> GMFNT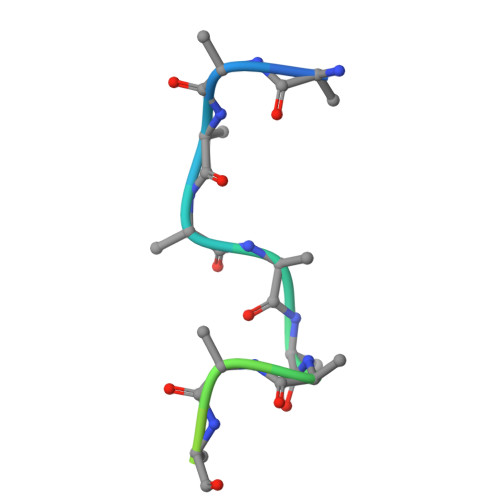TTMDDVYNYLFDDEDT Here we report, in contrast, on a naturally occurring mutation of an otherwise invariant residue in the β-glucosidase BglM-G1 that balances a trade-off between structural stability and enzyme activity. β-glucosidases are enzymes hydrolyzing β-glycosidic bonds in substrates ranging from glycosides, to glucosylated flavonoids, glucosylceramides, and oligosaccharides, releasing nonreducing terminal glucosyl residues (see Ketudat et al. for a comprehensive review). They are also one of the key enzymes in the bioconversion of cellulosic material. The otherwise invariant arginine at position 75 changed to a histidine in this protein, while the other 36 amino acids deemed necessary for the function and structural integrity of members of this protein family remained unchanged. Our data indicate that the natural mutation to histidine at position 75 leads to the loss of an extensive electrostatic network, including a salt bridge in the active site region and implies that evolution of BglM-G1 traded a decrease in thermal stability for improved catalytic efficiency.

We, therefore, re-introduced arginine, replacing the histidine 75 in this enzyme, creating the BglM-G1 variant H75R. There was, however, a major difference in electrostatic interactions between the mutation site and the active site nucleophile. The naturally occurring histidine at position 75 in BglM-G1 formed only a single hydrogen bond with the backbone oxygen of threonine 116, while arginine at position 75 formed, in addition to hydrogen bond interactions with residues Gln163 and Thr116, a salt bridge with the catalytic nucleophile glutamate at position 349 Fig. 2 CD spectroscopic analysis and X-ray crystal structure of BglM-G1 and its H75R variant. Because the crystal structure showed that arginine at position 75 forms a strong electrostatic interaction with the active nucleophile glutamate 349, this should lead to a more rigid substrate binding site in the variant. Asparagine 163 and Glutamate 349 were the two residues that had electrostatic interactions with both the inhibitor and Arginine 75. We thus inspected the B-factor of the atoms in the side chain of these two amino acids. A higher B-factor indicates higher flexibility in the crystal. The lower B-factors of residues Asparagine 163 and Glutamate 349 in the substrate binding site of BglM-G1’s H75R variant indeed suggest that the higher Km could be the result of a lower conformational flexibility caused by the stabilizing effect of the electrostatic network formed by Arginine 75.

>MHHHHHHENLYFQGHMKKWGDMFTWGVSTSSYQIEGAANQGGRGPSIWDTFSKIPGAVANGDNGDVACDHYHRYNEDLDLMKWLGVGAYRFSIAWPRVIPSGYGALNKEGMDFYDRLIDGALERGITPWPTLYHWDLPQSLQDKGGWNNRDCAYWFAEYSQKMAEAFSDRLKNWITINEPFCSAWLGHLYGVMAPGIKDLKTGINASHHLLLGHGLATKAIREVSSELKVGITLNFTPAITLGESSEDKLAVELADGFDNRWFGDPVFKAKYPEDIVKAFGKEVPIHPGDMEIISTPLDYLGLNYYFRQTVEYDATAKPLPYKQVTAPNVERTGMGWEVHAQSFTELLERVSKEYKPKEIFITENGSAWDDEVVDGKVDDPNRVSYLERHLDAMFAAKNKGVPISGYFAWSLIDNFEWAYGYAKRFGIIYVDYQTQKRIPKSSAYYYQKRIKES[3x]+/-METHYL 4-(AMINOIMINOMETHYL)-BETA-[3- INH (AMINOIMINO)PHENYL]BENZENE PENTANOATE 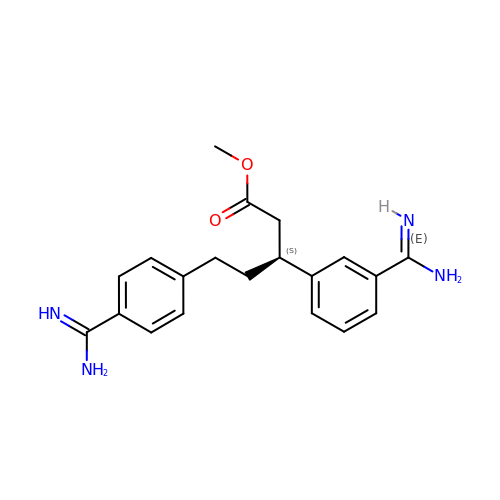| C20 H24 N4 O2 | PVALLOSAENRPQO-INIZCTEOSA-N>[5x]MGRAHKETLDKLTNAAINKINLLNTSKVKYLVSSAFAGLYVGIGILLIFTIGGLLTDAGSPMTKIVMGLSFAIALSLVIMTGTELFAGNNMVMSAGMLNKGVSIKDTSKIWAYSWVGNLIGALVLGIIFVGTGLVDKGPVAEFFANTAASKASMPFTALFFRGILCNILVCVSVLCSFRTNSDTAKIIMIFLCLFAFITSGFEHSVAN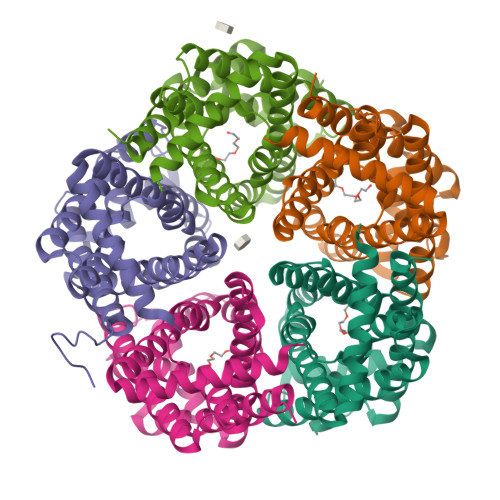MTIYSVSLFSPTISTVTIGGAIYNLVAVTLGNIVGGALFMGLGTYILGKEKLNAAAENLY> AEPPV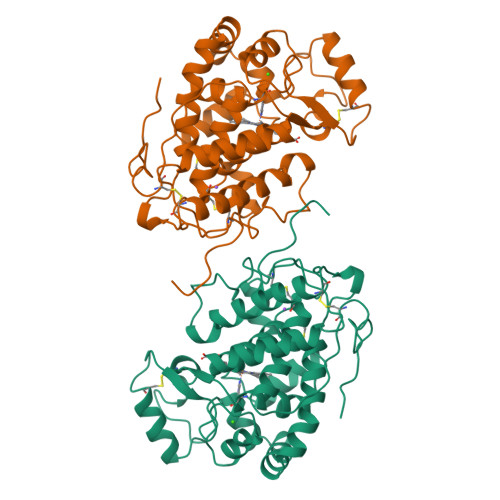APGLSFDFYWQTCPRAESIVREFVQEAVRKDIGLAAGLLRLHFHDCFVQGCDASVLLDGSATGPGEQQAPPNLTLRPSAFKAVNDIRDRLERECRGAVVSCSDILALAARDSVVVSGGPDYRVPLGRRDSRSFASTQDVLSDLPGPSSNVQSLLALLGRLGLDATDLVTISGGHTIGLAHCSSFEDRLFPRPDPTISPTFLSRLKRTCPAKGTDRRTVLDVRTPNVFDNKYYIDLVNREGLFVSDQDLFTNAITRPIVERFAQSQQDFFEQFGVSIGKMGQMRVRTSDQGEVRRNCSVRNPGPG>[2x]RWRAEGTSAHLRDIFLGRCAEYRALLSPEQRNKDCTAIWEAFKVALDKDPCSVLPSDYDLFITLSRHSIPRDKSLFWENSHLLVNSFADN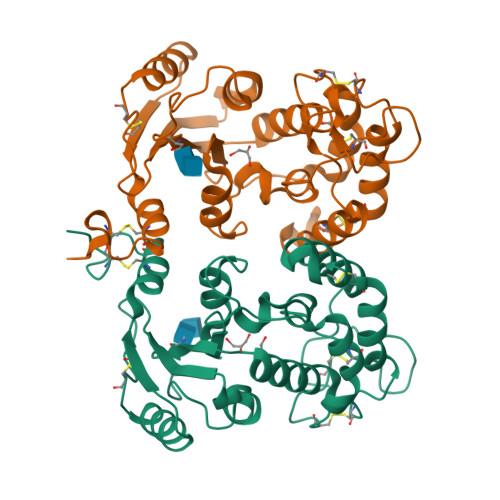TRRFMPLSDVLYGRVADFLSWCRQKADSGLDYQSCPTSEDCENNPVDSFWKRASIQYSKDSSGVIHVMLNGSEPTGAYPIKGFFADYEIPNLQKEKITRIEIWVMHEIGGPNVESCGEGSMKVLEKRLKDMGFQYSCINDYRPVKLLQCVDHSTHPDCALKSAAAATQRKAPSLY> AESLPDLKIEKLDEGVYVHTSFEEVNGWGVVPKHGLVVLVNAEAYLIDTPFTAKDTEKLVTWFVERGYKIKGSISSHFHSDSTGGIEWLNSRSIPTYASELTNELLKKDGKVQATNSFSGVNYWLVKNKIEVFYPGPGHTPDNVVVWLPERKILFGGCFIKPYGLGNLGDANIEAWPKSAKLLKSKYGKAKLVVPSHSEVGDASLLKLTLEQAVKGLNESKKPSKPSN

Production of metallo-β-lactamases (MBLs), which hydrolyze carbapenems, is a cause of carbapenem resistance in Enterobacteriaceae. The genes encoding MBLs, including IMP, NDM, and VIM types, have become widely prevalent via bacterium-specific transferable genetic apparatuses such as plasmids. We report here that sulfamoyl heteroarylcarboxylic acids (SHCs) can competitively inhibit the globally spreading and clinically relevant MBLs (i.e., IMP-, NDM-, and VIM-type MBLs) at nanomolar to micromolar orders of magnitude. X-ray crystallographic analyses revealed the inhibition mode of SHCs against MBLs; the sulfamoyl group of SHCs coordinated to two zinc ions, and the carboxylate group coordinated to one zinc ion and bound to positively charged amino acids Lys224/Arg228 conserved in MBLs.

Lineweaver-Burk plots demonstrated that SFC behaved as a competitive inhibitor with a submicromole-level Ki value for IMP-1 (0.22 μM) and micromole-level Ki values for NDM-1 and VIM-2 (9.82 μM and 2.81 μM, respectively). We carried out X-ray crystallographic analyses of IMP-1–SFC complexes. The overall structure of IMP-1–SFC complexes is shown in Fig. 3A; one SFC molecule was found to bind to the active site, scaffolding two zinc ions (Zn1 and Zn2). The sulfamoyl and carboxylate groups of SFC were clearly assigned with respect to the electron density observed. The details of the mode of binding of SFC to IMP-1 are revealed in an enlarged image, wherein the nitrogen atoms of the sulfamoyl group can be seen to located nearly equidistantly and to be coordinated with Zn1 and Zn2 (2.0 Å), which is where the hydroxyl anion for a nucleophilic attack was originally located in the native IMP-1 structure. Asp120 forms hydrogen bonds with the sulfamoyl group of SFC (2.8 Å), and the carbonyl oxygen of the sulfamoyl group is also hydrogen bonded to the nitrogen atom of the Asn233 side chain (2.9 Å). The spatial position of the Asn233 side chain shifted toward the zinc ions after the introduction of SFC. The carboxylate oxygen O1 of SFC coordinates with Zn2 (2.1 Å), and O2 interacts with the amide of Asn233 (2.9 Å) in the protein backbone and amino group of Lys224 (3.0 Å), which are conserved across B1 MBLs. Additionally, the methyl group (C6) at the 2-position of SFC is stacked in the cavity between Trp64 and His263, and this methyl moiety is likely stabilized via CH/π interactions through Trp64 and His263.2-[(1R)-1-methylpropyl]-4,5-dihydro-1,3-thiazole | C7 H13 N S | 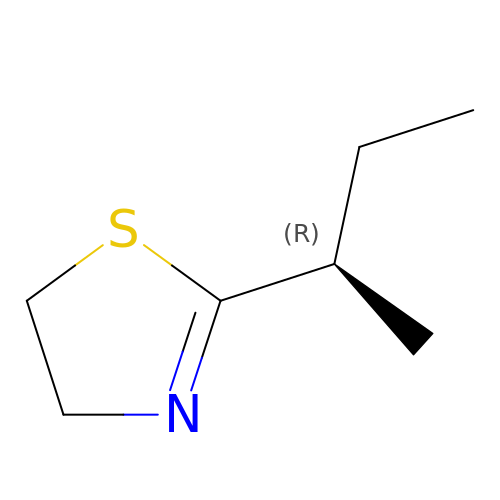SAWWKXMIPYUIBW-ZCFIWIBFSA-N>MDRYGVLAYHSVVDDTAAKEEKQYFPQTISANLLISHFNWLKDNGYNVVSWQQIIDAENGKSTLPEKAVVLSFDDGYATMYNVIYPILKAYNYPAVFAPVSSWLDTPVNQLIPYANIKLPRNVFVTWDQVREMEQSGLVEIASHTDNLHHGVRANPAGSQLPAVVAPEYKNNRYESKTEYKNRLVQDFSRSSKSIQRQIGKKPRIMVWPYGQFNDVAIDAAKQSGMTHHFALGQKIINKIGDRYVGRLLIDTETGFSTIKNFLDGVDDESK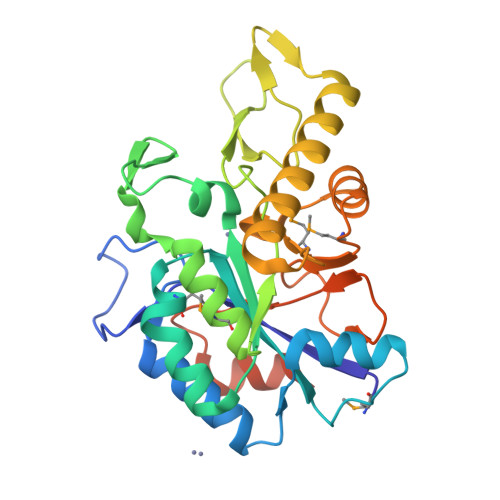LMRHHHHHH[2x]>MSDSTPKTPRGFVVHTAPVGLADDGRDDFTVLASTAPATVSAVFTRSRFAGPSVVLCREAVADGQARGVVVLARNANVATGLEGEENAREVREAVARALGLPEGEMLIASTGVIGRQYPMESIREHLKTLEWPAGEGGFDRAARAIMTTDTRPKEVRVSVGGATLVGIAKGVGMLEPDMATLLTFFATDARLDPAEQDRLFRRVMDRTFNAVSIDTDTSTSDTAVLFANGLAGEVDAGEFEEALHTAALALVKDIASDGEGAAKLIEVQVTGARDDAQAKRVGKTVVNSPLVKTAVHGCDPNWGR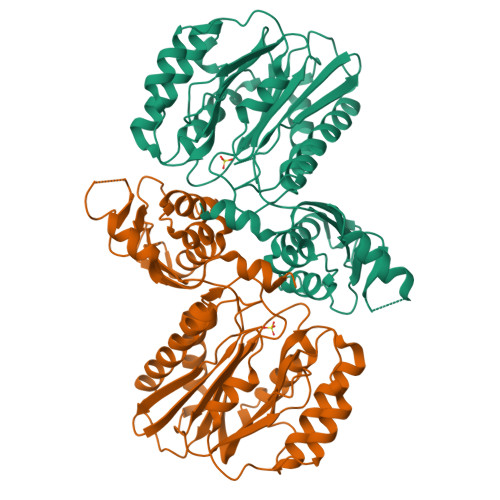VAMAIGKCSDDTDIDQERVTIRFGEVEVYPPKARGDQADDALRAAVAEHLRGDEVVIGIDLAIADGAFTVYGCDLTEGYVRLNSEYTT[4x]> XEAQT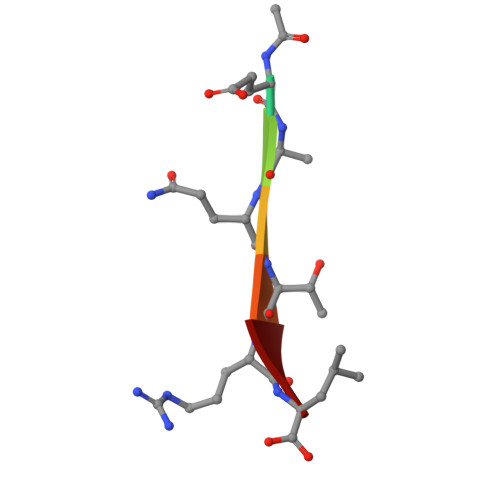RL> DITQQAKDIGAGPVASCFTTRMSPPQQICLNSV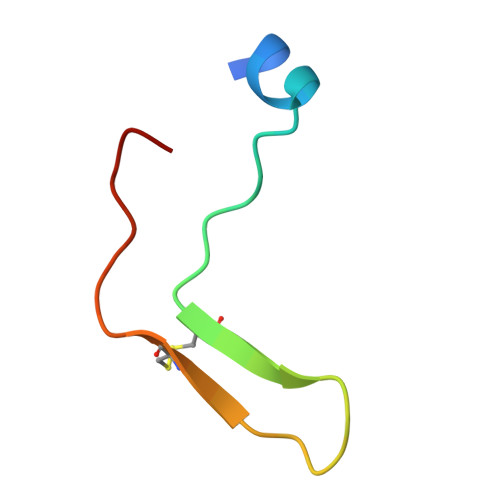VNTALS>[2x]SGAMDKIKYSPEA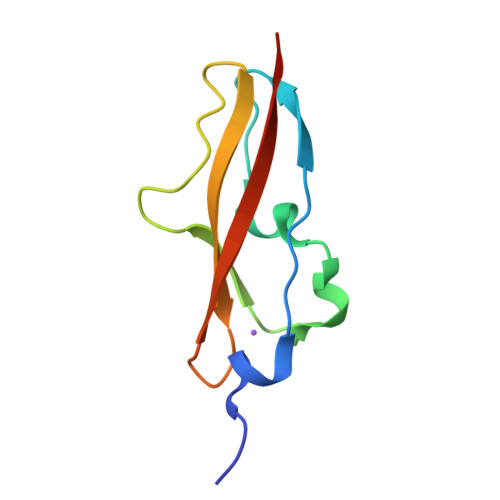KHRTVEQHAELDAKDSIANTDELPSNSTYNWKNGHKPDTSTSGEKDGIVEVHYPDGTVDDVNVKVTVTSKKT> MITILDYLFLLDLNDDLTRKAVFEQVIIFIFIYCTMNFLAWSTVVELIWPTHFFNRRHSSSQEF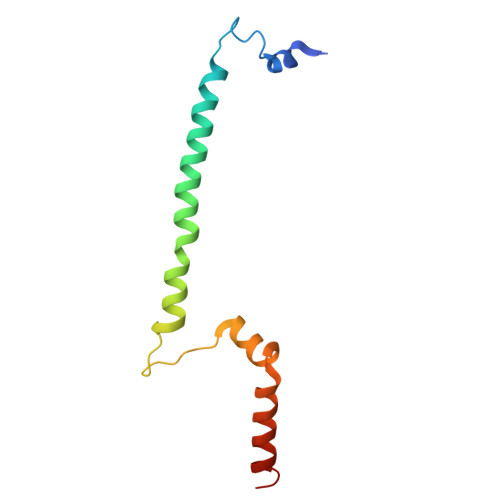IRFRTYTEVLLKISAYNDFFYVLNNYYYNQKLILKN>[10x]MEALPLLAATTPDHGRHRR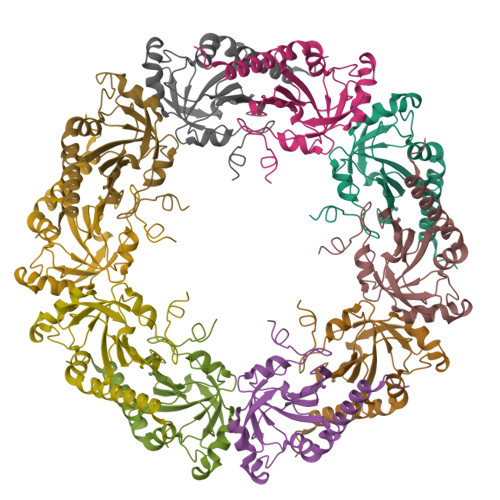LLLLPLLLFLLPAGAVQGWETEERPRTREEECHFYAGGQVYPGEASRVSVADHSLHLSKAKISKPAPYWEGTAVIDGEFKELKLTDYRGKYLVFFFYPLDFTFVCPTEIIAFGDRLEEFRSINTEVVACSVDSQFTHLAWINTPRRQGGLGPIRIPLLSDLTHQISKDYGVYLEDSGHTLRGLFIIDDKGILRQITLNDLPVGRSVDETLRLVQAFQYTDKHGEVCPAGWKPGSETIIPDPAGKLKYFDKLN> MLSTGPIMETLTLTVGSAFEIPGWKLRGEYPAGTTSHLVFTDAAGGTLGEFEGTVSAKEIHYLQAPDDVKNIPHGANFQLFVTYPSMQPQCLYFGTAIRKEPRYPLSTVVSPEDSAVQYKANFVGQYIGPMWKPMGNGWGSLGIHTHAL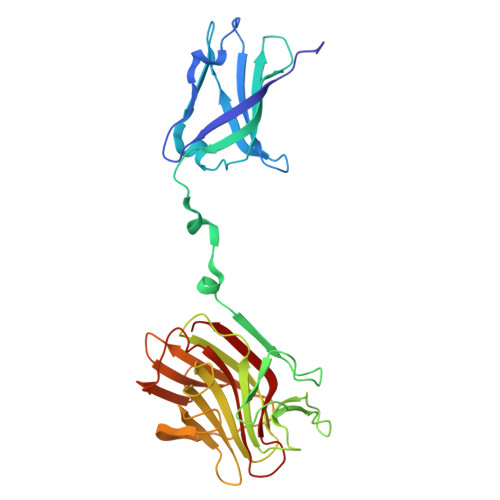ISEAPSMGPNYSLFSSAAARWLWSMNMDSVTIVVRVLNVGAGKFNVIVCADYQMQTYLGIQFETGISNNKVHVITGDGPLNWGYQGDAVNNTTANGDVYTIKYNDLLDTISCYKGTSLTPLIEASGLDVPHGEGFRYTGLAWNTALLSPGVEPTAWEAKDGV> GSHMPAAVSDADFATLEKTSGGRLGVCLWHPASGARYGHRMDERFPMCSTVK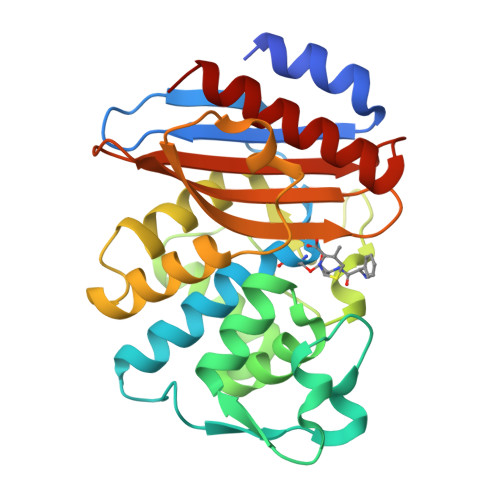FPLAAAILHRVDAGKLSLDQRVAVRQGDIISHSPFTERHVGKDMTVRDLCRATLIISDNAAANLLLPLIDGPAGLTAFLQAQGDRITVSARNQPELNHFAPGDPRDTTSPAAMAGNLQRFLLGDVLSPASRQQLADWLIDNQTGDARLRAGLPQGWRVGDKTGSNGQDTSNDIAALWPLAGGAPWLLSCYLQGSALDDDGRDGILRQVGELAGARLG5-[methyl-[(2-propoxypyridin-3-yl)methyl]amino]-2~{H}-indazole-3-carboxylic 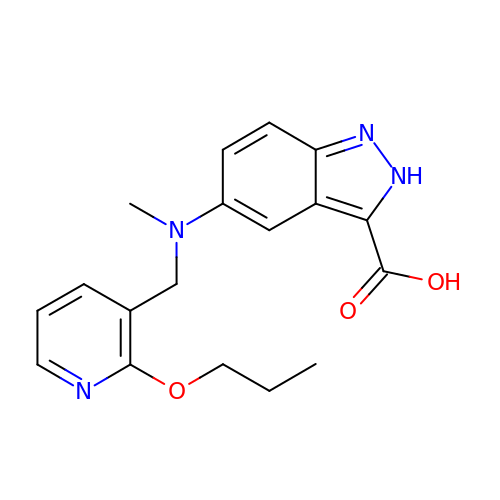acid | C18 H20 N4 O3 | RVGJIJTWOILHDF-UHFFFAOYSA-N>MVHYKLTYFAIRGAGECARQIFALADQEFEDVRLDKEQFAKVKPDLPFGQVPVLEVDGKQLAQSLAICRYLARQFGFAGKSTFDEAVVDSLADQYSDYRVEIKSFFYTVIGMREGDVEQLKKEVLLPARDKFFGFITKFLKKSPSGFLVGD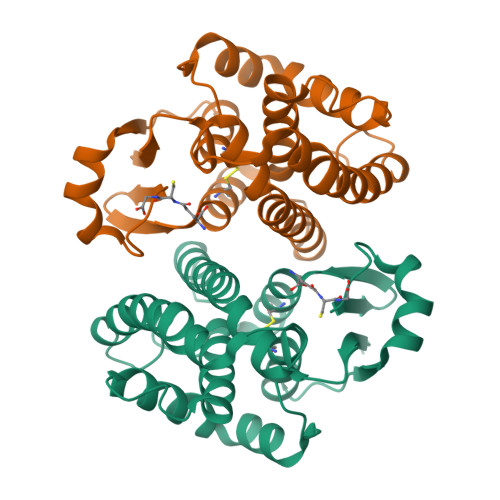SLTWVDLLVSEHNATMLTFVPEFLEGYPEVKEHMEKIRAIPKLKKWIETRPETLF[2x]>[12x]HHSQDPMLSKDIIKLLNEQVNKEMNSSNLYMSMSSWCYTHSLDGAGLFLFDHAAEEYEHAKKLIIFLNENNVPVQLTS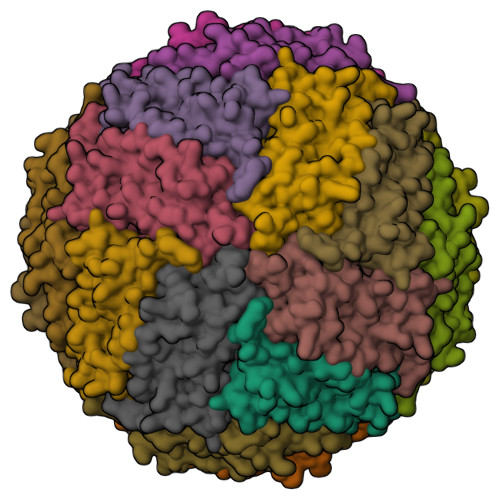ISAPEHKFEGLTQIFQKAYELEQHISESINNIVDHAIKSKDHATFNFLQWYVAEQHEEEVLFKDILDKIELIGNENHGLYLADQYVKGIAKSRKS> GTQPTFGFTVNWKFSESTTVFTGQCFIDRNGKEVLKTMWLLRSSVNDIGDDWKATRVGINIFTRLRTQKEGGSGGSARKCSLTGKWTNDLGSNMTIGAVNSRGEFTGTYITAVTATSNEIKESPLHGTQNTINKSGGSTTVFTGQCFIDRNGKEVLKTMWLLRSSVNDIGDDWKATRV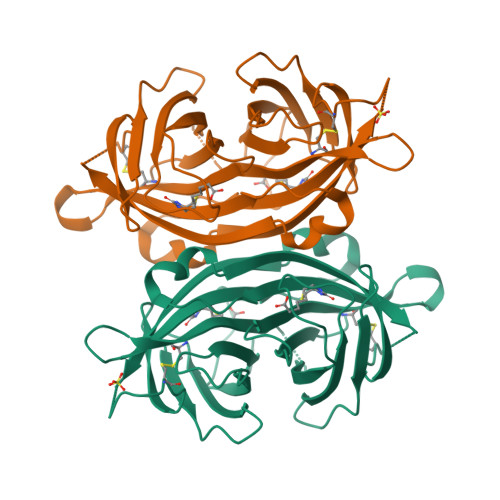GINIFTRLRTQKEGGSGGSARKCSLTGKWTNDLGSNMTIGAVNSRGEFTGTYITAVTATSNEIKESPLHGTQNTINKRTQPTFGFTVNWKFSE>[4x]MRLDVEQTSKLDRVRADYNVHYWSQGFYGIDDQGEMYVSPRSDNAHQIQLSKIVKQLEERQLNVPVLVRFPQILHQRVHSICDAFNQAIEEYQYPNKYLLVYPIKVNQQREVVDEILASQAQLETKQLGLEAGSKPELLAVLAMAQHASSVIVCNGYKDREYIRLALIGEKLGHKVFIVLEKMSELDLVLREAKSLGVTPRLGIRIRLASQGAGKWQASGGEKSKFGLSASQVLNVISRLKKENQLDTLQLVHFHLGSQMANIRDVRNGVNESARFYCELRTLGANITYFDVGGGLAIDYDGTRSQSSNSMNYGLVEYARNIVNTVGDVCKDYKQPMPVIISESGRSLTAHHAVLISNVIGTETYKPETVTEPEEDFPLLLNNMWRSWLNLH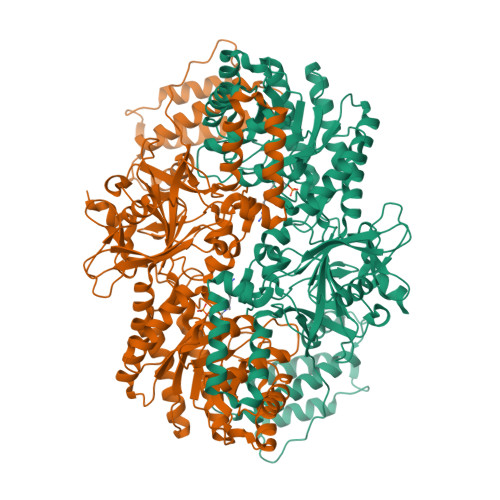NGTDARALIEIYNDTQSDLAEVHSQFATGVLTLEHRAWAEQTSLRIYYELNRLMSTKNRFHRPILDELSERLADKFFVNFSLFQSLPDSWGIDQVFPVLPLSGLQNAADRRAVMLDITCDSDGAIDAYVDGQGIESTLPVPAWNEDEPYLMGFFLVGAYQEILGDMHNLFGDTHSVVVNVGDQGEINIDFINEGDTVEDMMRYVHIDVDQIRKNYHSLVSQRVDQEEQQQILAELEQGLSGYTYLEDFLEHHHHHH>APITAYSQQTRGLLGCIITSLTGRDKNQVDGEVQVLSTATQSFLATCVNGVCWTVYHGAGSKTLAGPKGPITQMYTNVDQDLVGWPAPPGARSMTPCTCGSSDLYLVTRHADVIPVRRRGDSRGSLLSPRPVSYLKGSSGGPLLCPSGHVVGIFRAAVCTRGVAKAVDFIPVESMETTM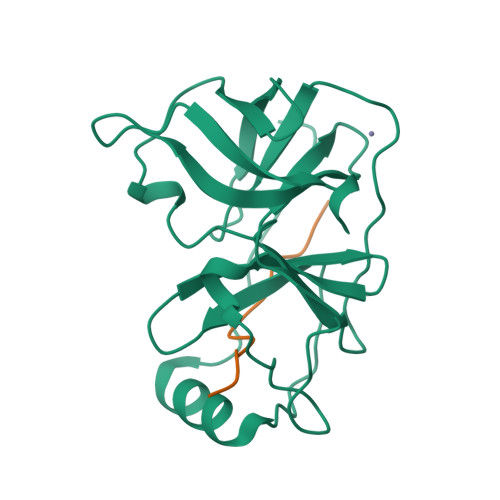RSPVFTDN[2x];>KGSVVIVGRIILSGRK[2x]Mitogen-activated protein kinase kinase kinase kinase 1 (MAP4K1) is a serine/threonine kinase that acts as an immune checkpoint downstream of T-cell receptor stimulation. MAP4K1 activity is enhanced by prostaglandin E2 (PGE2) and transforming growth factor beta (TGFβ), immune modulators commonly present in the tumor microenvironment. Therefore, its pharmacological inhibition is an attractive immuno-oncology concept for inducing therapeutic T-cell responses in cancer patients. Through its proline-rich domain, MAP4K1 binds to a diversity of adaptors in hematopoietic cells, including those involved in T-cell receptor (TCR), B-cell receptor, and cytokine-induced signaling. The function of MAP4K1 has been studied most extensively in the context of T-cell activation.

Through iterative structure–activity relationship (SAR) studies, optimization efforts led to the discovery of compound 38 (BAY-405), which is a highly potent and selective inhibitor of MAP4K1. BAY-405 displayed potent activity toward MAP4K1 in biochemical and cellular assays, with a ROCK2 selectivity ratio of 130 in the biochemical assay and an overall selectivity score of S = 0.080 (80%, 1 μM)27 against an external kinase panel consisting of 373 kinases, representing a significant improvement over compound 1 (BAY-755; S = 0.13). BAY-405 was confirmed as an ATP competitive active site inhibitor, as demonstrated by the fact that both kinase inhibitor (IC50 = 11 nM) and ATP binding competition assays (IC50 = 6.2 nM) rendered highly comparable IC50 values, and further supported by a prominent shift in IC50 value in a high ATP kinase activity assay (IC50 = 56 nM at 1 mM ATP). With respect to cellular activity, BAY-405 inhibited phosphorylation of SLP76 with submicromolar activity (IC50 = 0.63 μM). The X-ray structure of BAY-405 in complex with the kinase domain of human MAP4K1 shows an ATP-competitive binding mode, with the pyrrolopyridine anchoring the molecule to the hinge region via two classical hydrogen bonds. The trifluoromethyl-cyclopropyl moiety sits smoothly in the back pocket of the kinase, which remains in a DFG-in conformation. The central fluorinated phenyl ring (A-ring) is arranged perpendicular to the hinge binding heterocycle, with the conformation being stabilized by the o,o-disubstitution. The tip of the nucleotide binding loop folds back into the pocket, allowing for a π–π-stacking interaction of the A-ring with the side chain of Tyr28. While the oxazine moiety engages in a bidentate H-bond with the Asp101 carboxylic acid, the terminal tetrahydropyran ring in the spiro-ring system does not show any direct interactions with the crystallized kinase domain. BAY-405 enhances T-cell immunity and overcomes the suppressive effect of PGE2 and TGFβ.

> GMDVVDPDIFNRDPRDHYDLLQRLGGGTYGEVFKARDKVSGDLVALKMVKMEPDDDVSTLQKEILILKTCRHANIVAYHGSYLWLQKLWICMEFCGAGSLQDIYQVTGSLSELQISYVCREVLQGLAYLHSQKKIHRDIKGANILINDAGEVRLADFGISAQIGAELARRLEFIGTPYWMAPEVAAVALKGGYNELCDIWSLGITAIELAELQPPLFDVHPLRVLFLMTKSGYQPPRLKEKGKWSAAFHNFIKVTLTKSPKKRPSATKMLSHQLVSQPGLNRGLILDLLDKLKNPGKGPSIGDIEDEE> 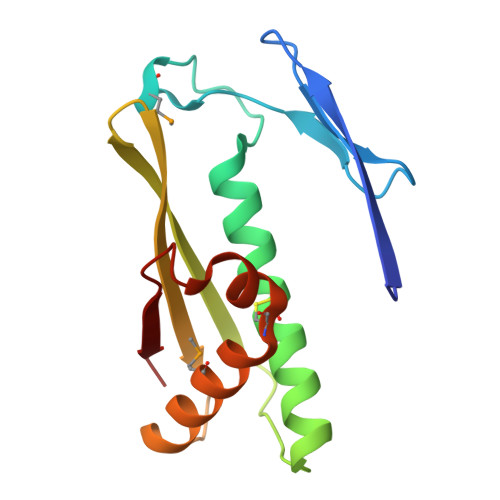MANVYTAEATATGGRAGTTRSSDDRLNLDLSVPAEMGGDGGPGTNPEQLFAAGYAACFQGALGVVSRRQKIDVPADSTITARVGLQKAGLAFALDVELEGHFPGLSREQAEGLMHAAHEVCPYSAATRNNVDVRLKVRE>[2x]GSMEKSMSPFVKKHFVLVHTAFHGAWCWYKIVALMRSSGHNVTALDLGASGINPKQALQIPNFSDYLSPLMEFMASLPANEKIILVGHALGGLAISKAMETFPEKISVA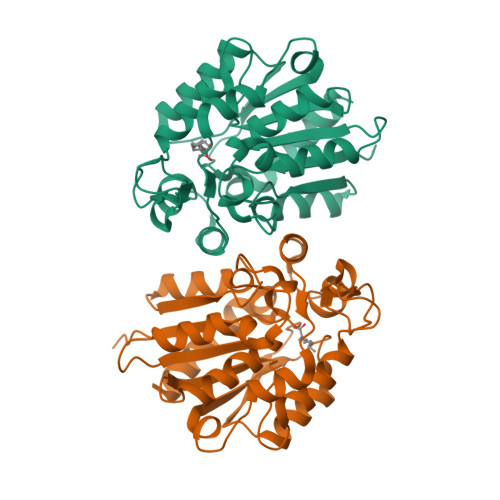VFLSGLMPGPNIDATTVCTKAGSAVLGQLDNCVTYENGPTNPPTTLIAGPKFLATNVYHLSPIEDLALATALVRPLYLYLAEDISKEVVLSSKRYGSVKRVFIVATENDALKKEFLKLMIEKNPPDEVKEIEGSDHVTMMSKPQQLFTTLLSIANKYK>[4x]GPHMRTISYSEARQNLSATMMKAVEDHAPILITRQNGEACVLMSLEEYNSLEETAYLLRSPANARRLMDSIDSLKSGKGTEKDIIE;>[2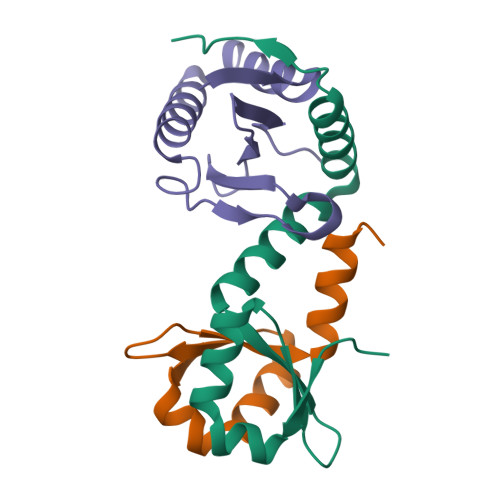x]MKLIWSEESWDDYLYWQETDKRIVKKINELIKDTRRTPFEGKGKPEPLKHNLSGFWSRRITEEHRLVYAVTDDSLLIAACRYHY> MALLNFQKPDKVIMIDSTDFEGKFEFRPLEPGYGLTVGNALRRVLLSSLEGFAITSVRIDGVEHEFSVVPGVVEDVTEIILNLKQVRFKRQIDDVESETVSISVSGKEQLTAGDFQKFISGYQVLNPDLVICNMGPKVSINMEIVIEKGRGYVPAEENKKSNAPLGSIAVDSVYTPVKNVKYSIENYRVEQKTDYEKLVFEIITDGSIHPKDALTEAAKVLIHHFMLFSDERITLEADEIAQTETYDEESLHMRQLLKTKLVDMDLSVRALNCLKAAEVDTLGDLVSFNKNDLMK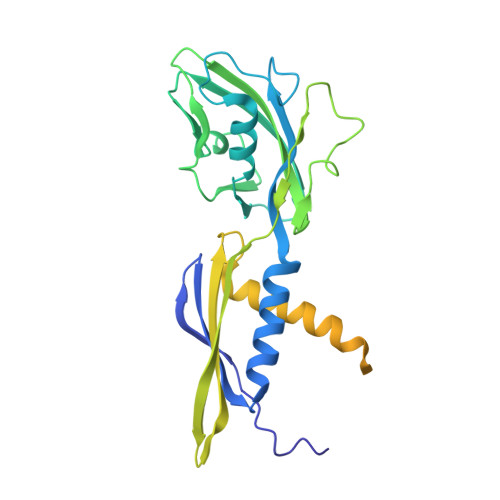FRNFGKKSLTELEELVINKGLQFGMDLSKYKLDKD>[4x]GSSHHHHHHMSGENLYFQGASAAIVTDTGGVDDKSFNQSAWEGLQAWGKEHNLSKDNGFTYFQSTSEADYANNLQQAAGSYNLIFGVGFALNNAVKDAAKEHTDLNYVLIDDVIKDQKNVASVTFADNESGYLAGVAAAKTTKTKQVGFVGGIESEVISRFEAGFKAGVASVDPSIKVQVDYAGSFGDAAKGKTIAAAQYAAGADIVYQVAGGTGAGVFAEAKSLNESRPENEKVW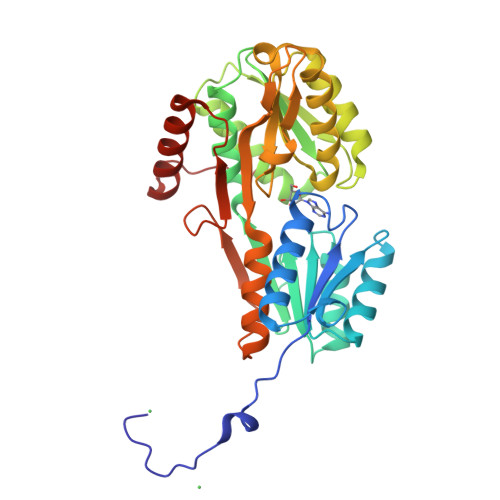VIGVDRDQEAEGKYTSKDGKESNFVLVSTLKQVGTTVKDISNKAERGEFPGGQVIVYSLKDKGVDLAVTNLSEEGKKAVEDAKAKILDGSVKVPEK>SRRTYTLT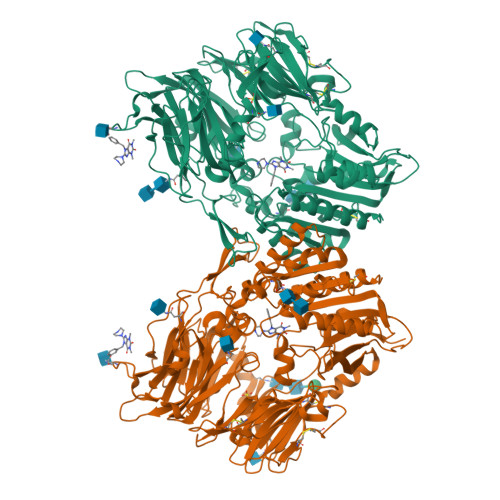DYLKSTFRVKFYTLQWISDHEYLYKQENNILLFNAEYGNSSIFLENSTFDELGYSTNDYSVSPDRQFILFEYNYVKQWRHSYTASYDIYDLNKRQLITEERIPNNTQWITWSPVGHKLAYVWNNDIYVKNEPNLSSQRITWTGKENVIYNGVTDWVYEEEVFSAYSALWWSPNGTFLAYAQFNDTEVPLIEYSFYSDESLQYPKTVRIPYPKAGAENPTVKFFVVDTRTLSPNASVTSYQIVPPASVLIGDHYLCGVTWVTEERISLQWIRRAQNYSIIDICDYDESTGRWISSVARQHIEISTTGWVGRFRPAEPHFTSDGNSFYKIISNEEGYKHICHFQTDKSNCTFITKGAWEVIGIEALTSDYLYYISNEHKGMPGGRNLYRIQLNDYTKVTCLSCELNPERCQYYSASFSNKAKYYQLRCFGPGLPLYTLHSSSSDKELRVLEDNSALDKMLQDVQMPSKKLDVINLHGTKFWYQMILPPHFDKSKKYPLLIEVYAGPCSQKVDTVFRLSWATYLASTENIIVASFDGRGSGYQGDKIMHAINRRLGTFEVEDQIEATRQFSKMGFVDDKRIAIWGWSYGGYVTSMVLGAGSGVFKCGIAVAPVSKWEYYDSVYTERYMGLPTPEDNLDYYRNSTVMSRAENFKQVEYLLIHGTADDNVHFQQSAQLSKALVDAGVDFQTMWYTDEDHGIASNMAHQHIYTHMSHFLKQCFSLP[4x]>MNWSKAINFQPFMLETRPPLTTIPIMDQLVEIGERSNQKWSMTDRLFFAIRKINPIFVTSSQIPSKFDYTILQMPTQLIASLKETLLFLAFSYYLREYQDKVGQMKFYPVAMKNMIPIVNYLKDRVHNNFDTTLEQAYRQNVVHTLSASDAFDLLSGMIATTRLDLIQRTRICPELLNVLNKMSFILIYAPNRPSILSWKNQS[2x];>[2x]MASTTRLVNDRKQLEQQVKDDARILADARGLNITTVANDSATGGQAIRNVGPNDEATIKALDNVIKQIEALSVIVNRSEKADDAQILGPNTYKQLLEHLFSPEENVYILLPIQAYTGGVIDRRDASFSNFAYSIASKLMMELSAATHNKIFTDYTRIAASALGPEISTEGMPLFSLIESLELTEAETSRLPVIQDSMVIQKSTATVGNAQQGISTINIKRVPFVGSAFQQVIDQLLWEYSTTSLTTKEQRRQRITEMVNDRRIMIQKLTLAEKPQVMRHV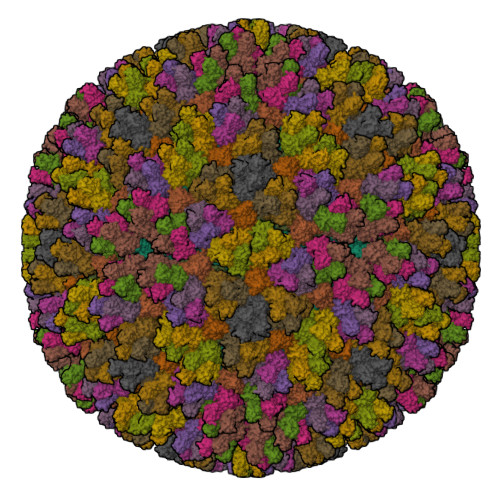TTEINNDLFFKMSPVAQLYIYHLDRAFLDGVGFTPLAEKQQQLQLQLKTNILTANLIRSAINGMNTESNLEVAIKMMQAAQLHRASIEIAFPMNVSLSPEIIVQCFIVWMSIPEQLLSDRSNFIIAAVIWAGFSADDSYADIMRRSARASDRQNYDIIKAALSSRKFKLPRASTTLFDENEPVVRRYQIGRVYAPFPVDRYGSPVYSNCTKVELASDYNAEGFTIRKDDFRALQAVLRIDEDRAADMFTTLRIMISSIPAVWYDAEVVHYPHTAVELEQLAAYGLTGAYPRTNHSVDTIVKTVNNISATYSTIAQMLSTIDLDPTRYGTSESIDKFKIAWENVESVLNMEGNDFVKTIMYAYEDNFPKKDFYMMLKQIASDGQGAHPIAAAIDQLRTIVYREPERFGYIDSVILTHNPDVDTAYNRFFHLHPIVTNQPSNTIKNAQLWNEMRLEQQVEHIKAGPVRIIGPFHVTYNYLSEEEDMPATSHIIMKDNMILNDHLTFNFVKRERRNNKKRVSSFRYKAVEMYVAVRISRFQLEVLRDLHDLVRSRTYLDVSKSPLATTPIRVVEYVR;>MNLEINNFAPAISSIGSQLCSLSAQKLLTCRKQYGNGAKSFEEFYAEIGGIIGMMGINSQTPSGIREAIYRLYQSAFLFGDIFPESFGIQNTQNIKPPPGFTAPAKKLEVVLPQGGAFDLIYNNGEIRVTTTRNVQAGDLVCTVTFPIQGSVIATRNCHVNEIGGQLTTTRPEIIASVPMPARTVIVASFDAIEIGYGEGDDLFAIGIAILSNRFNGQITPMSRHNYMTQMFANLPANMSERDSSAVLHFAQAAPVVLGMMERLTGAPKWVLDY[13x]> MNHPLFTEGTYQAEVMENSPAGTPLTVLNGPILALDADEDVYAVVTYQLLGTH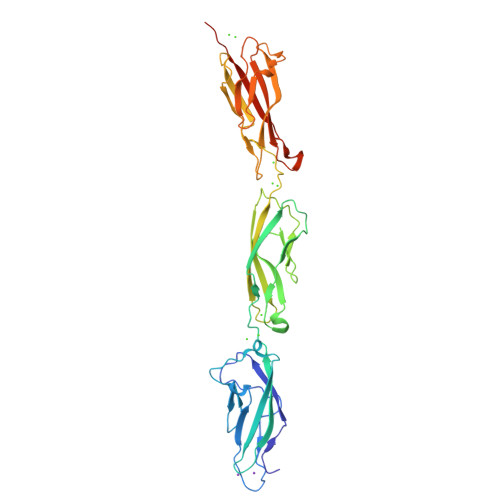SDLFVIDNSTGVVTVRSGIIIDWEAFSPPFLELLLLAEDIGQLNGTAHLFITILDDNDNWPTFSPPTYTVHLLENCPPGFSVLQVTATDEDSGLNGELVYRIEAGAQDRFLIHPVTGVIRVGNATIDREEQESYRLTVVATDRGTVPLSGTAIVTILIDDINDSRPEFLNPIQTVSVLESAEPGTIIANVTAIDLDLNPKLEYHIISIVAKDDTDRLVPDQEDAFAVNINTGSVMVKSPLNRELVATYEVTLSVIDNASDLPEHSVSVPNAKLTVNILDVNDNLEHHHHHH>GRVYLVGAGPGDPELLTLKAYRLLKEAPVVLYDRLVDERVLALAPGEKVYVGKEEGESEKQEEIHRLLLRHARAHPFVVRLKGGDPMVFGRGGEEVLFLLRHGVPVEVVPGVTSLLASGLPLTHRGLAHGFAAVSGVLEGGGYPDLRPFARVPTLVVLMGVGRRVWIAKELLRLGRDPREPTLFVERASTPKERRVHARLEEVAEGKVEVRPPALWILGE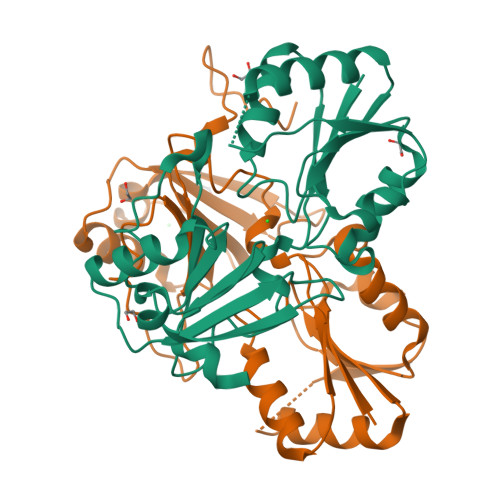VVRVFAEKEAPVDALALGG[2x]>MEQRRLASTEWVDIVNEENEVIAQASREQMRAQCLRHRATYIVVHDGMGKILVQRRTETKDFLPGMLDATAGGVVQADEQLLESARREAEEELGIAGVPFAEHGQFYFEDKNCRVWGALFSCVSHGPFALQEDEVSEVCWLTPEEITARCDEFTP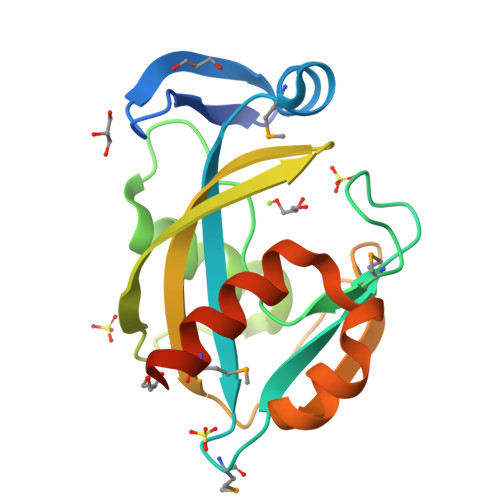DSLKALALWMKRNAKNEAVETETAE[3x]> MPKHGKRYRALLEKVDPNKIYTIDEAAHLVKELATAKFDETVEVHAKLGIDPRRSD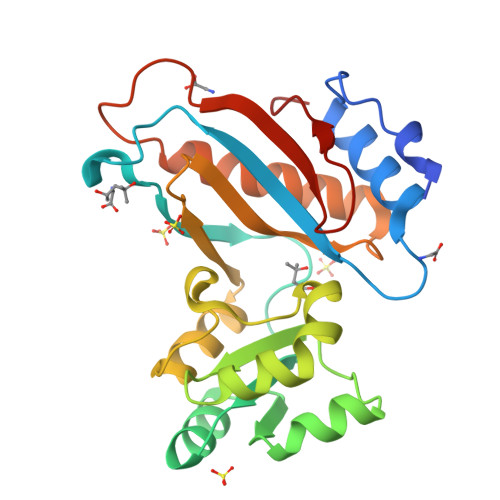QNVRGTVSLPHGLGKQVRVLAIAKGEKIKEAEEAGADYVGGEEIIQKILDGWMDFDAVVATPDVMGAVGSKLGRILGPRGLLPNPKAGTVGFNIGEIIREIKAGRIEFRNDKTGAIHAPVGKASFPPEKLADNIRAFIRALEAHKPEGAKGTFLRSVYVTTVMGPSVRINPHS> GSHMSDSKEVPSLPFLRHLLEELDSHEDSLLLFLCHDAAPGCTTVTQALCSLSQQRKLTLAALVEMLYVLQRMDLLKSRFGLSKEGAEQLLGTSFLTRYRKLMVCVGEELDSSELRALRLFACNLNPSLSTALSESSRFVELVLALENVGLVSPSSVSVLADMLRTLRRLDLCQQLVEYE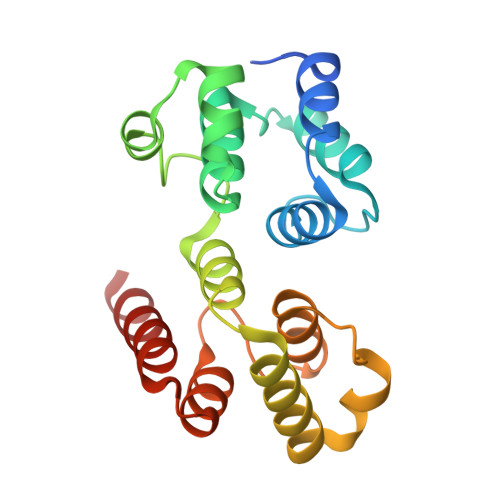QQEQAR>GAMDQRMYSRRSLYHTRTKDLKDFIRVHRLPKALAQRMLECFQTTWSVNNGIDVSELLKDFPDELRADIAMHLNKELLQLPLFESASRGCLRSLSLIIKTSFCAPGEFLIRQGDALQAIYFVCSGSMEVLKDNTVLAILGKGDLIGSDSLTKEQVIKTNANVKALTYCDLQYISLKGLRE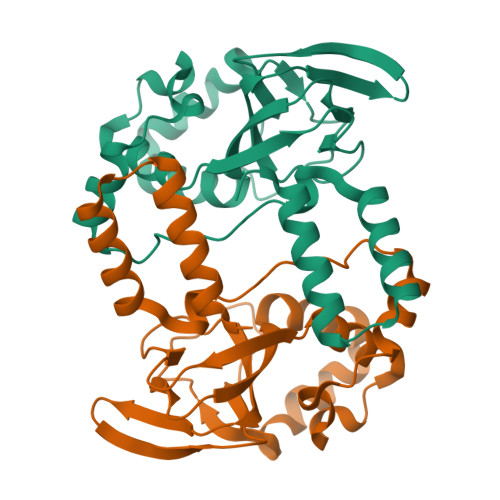VLRLYPEYAQKFVSEIQHDLTYNLREGSGADL[4x]> DCHLSDMLQQLHSVNASKPSERGLVRQEEAEDPACIPIFWVSKWVDYSDKYGLGYQLCDNSVGVLFNDSTRLILYNDGDSLQYIERDGTESYLTVSSHPNSLMKKITLLKYFRNYMSEHLLKAGANITPREGDELARLPYLRTWFRTRSAIILHLSNGSVQINFFQDHTKLILCPLMAAVTYIDEKRDFRTYRLSLLE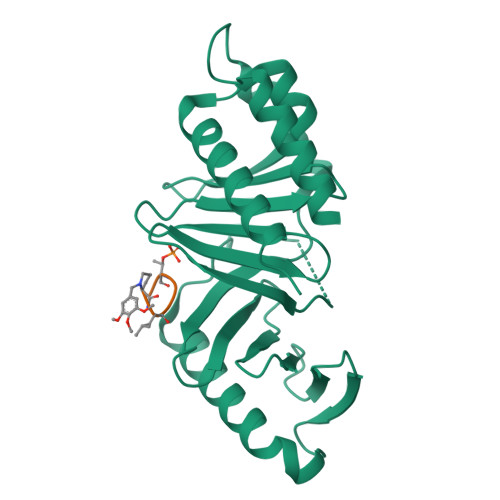EYGCCKELASRLRYARTMVDKLLSSRS>MITKSNEFWTPKRLLETDDRIFLVVGGRGVGKTFNVTGEALDDLFFNNVSMVYLRRLGVEIDELEKNNFITEEMLRVYFGNRFSDFNADESKQIMRFSIDGAIHEIKAIRNKIFFDDRCIVYFIALSRAGHVKSNNYPDVKYLVFDEVIIDRSIMPNARYIRNEFTVLLNLIETIKRKREDFYLFMLSNVGENFNPIFAGLGYYLTHEDIKKGFVKREDYCVQFVENKQEELNMTDPFVRLGAKNRDFSNSKTNAFENIRTPYFKHYGKKPKLLVKYDRQYLGIAERKIPSGLEYYYQVYKTLDGLENITVFNNNFDTLMEDEVFLEETQ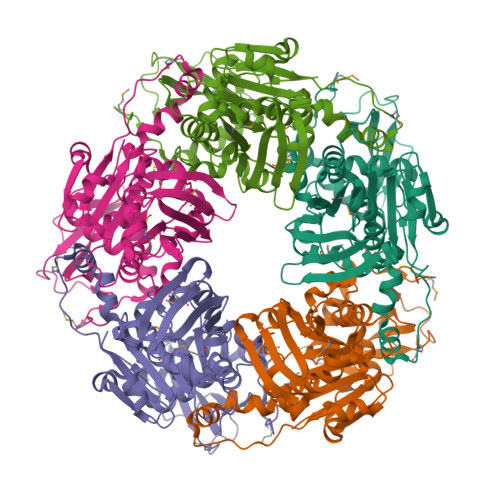LKKKFKTYFELFQQNMVYHESPETFLEWSKFVYALKLEHHHHHH[5x]> MKVGQDKVVTIRYTLQVEGEVLDQGELSYLHGHRNLIPGLEEALEGREEGEAFQAHVPAEKAYGPHDPEGVQVVP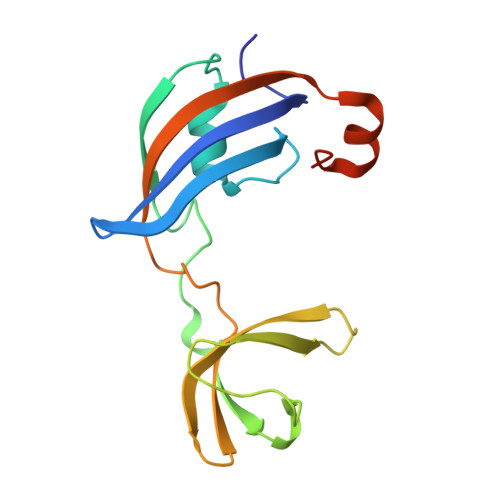LSAFPEDAEVVPGAQFYAQDMEGNPMPLTVVAVEGEEVTVDFNHPLAGKDLDFQVEVVKVREATPEELLHGHAHPGHHHHHH>GAMGASGKIKISTPYNLTKRMMMPMLNGFMSQYPEINIELTTESNADQLDPTEWDVIFRVGPQRDSSLIARKIGSVKDILVASPEYVNAHPMPTHAEDLHDHFLLKGHPLLKWTLINSKGETVVNVDRGRFQANALNVVRSACSEGLGITLMPDVMIKEYIADGSLVRILPDWSANPRDIYMLYNHKDHLPEK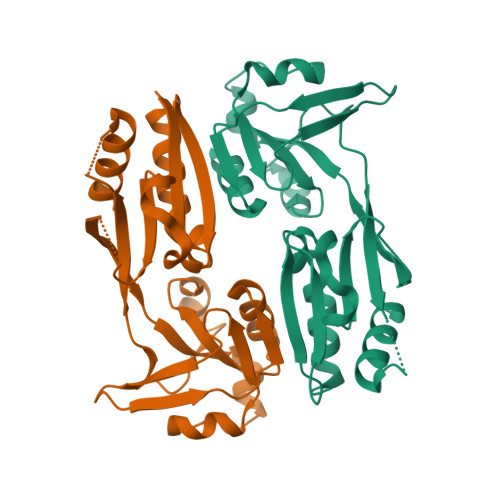VRLFIDYVIAYNIH[6x]PHOSPHORYL-HEXAETHYLENE GLYCOL | 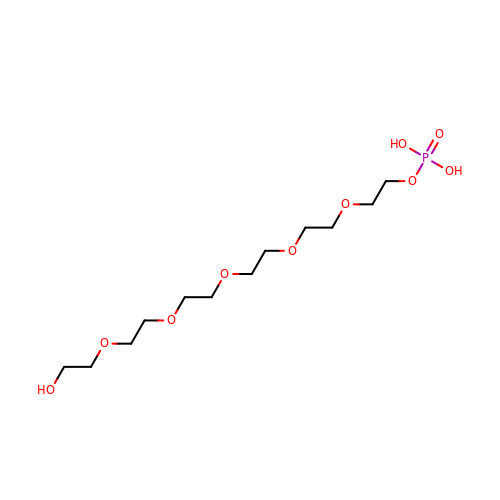C12 H27 O10 P | PTMCGHPIYOSATH-UHFFFAOYSA-N> DRWGSELPAQKWWHTGALYRIGDLQAFQGHGAGNLAGLKGRLDYLSSLKVKGLVLGPIHKNQKDDVAQTDLLQIDPNFGSKEDFDSLLQSAKKKSIRVIL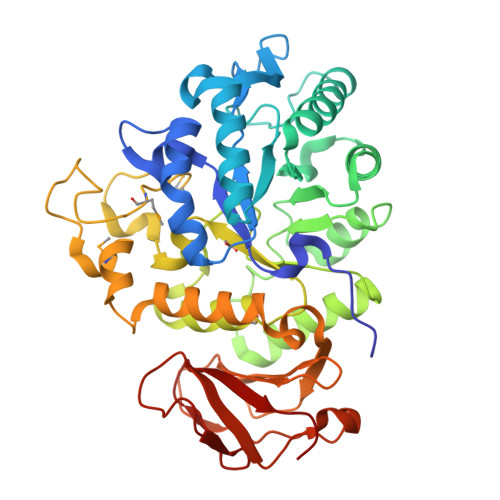DLTPNYRGENSWFSTQVDTVATKVKDALEFWLQAGVDGFQVRDIENLKDASSFLAEWQNITKGFSEDRLLIAGTNSSDLQQILSLLESNKDLLLTSSYLSDSGSTGEHTKSLVTQYLNATGNRWCSWSLSQARLLTSFLPAQLLRLYQLMLFTLPGTPVFSYGDEIGLDAAALPGQPMEAPVMLWDESSFPDIPGAVSANMTVKGQSEDPGSLLSLFRRLSDQRSKERSLLHGDFHAFSAGPGLFSYIRHWDQNERFLVVLNFGDVGLSAGLQASDLPASASLPAKADLLLSTQPGREEGSPLELERLKLEPHEGLLLRFPYAA>[2x]MDFKTVMQELEALGKE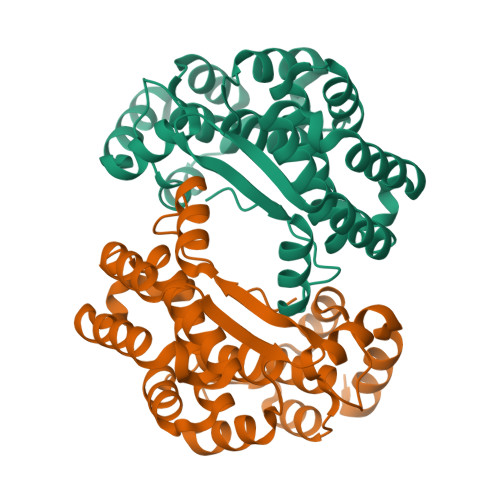RTKKIYISNGAHEPVFGVATGAMKPIAKKIKLNQELAEELYATGNYDAMYFAGIIADPKAMSESDFDRWIDGAYFYMLSDYVVAVTLSESNIAQDVADKWIASGDELKMSAGWSCYCWLLGNRKDNAFSESKISDMLEMVKDTIHHSPERTKSAMNNFLNTVAISYVPLHEKAVEIAKEVGIVEVKRDNKKSSLLNASESIQKELDRGRLGFKRKYVRC>[4x]MNKHVNKVALIGAGFVGSSYAFALINQGITDELVVIDVNKEKAMGDVMDLNHGKAFAPQPVKTSYGTYEDCKDADIVCICAGANQKPGETRLELVEKNLKIFKGIVSEVMASGFDGIFLVATNPVDILTYATWKFSGLPKERVIGSGTTLDSARFRFMLSEYFGAAPQNVCAHIIGEHGDTELPVWSHANVG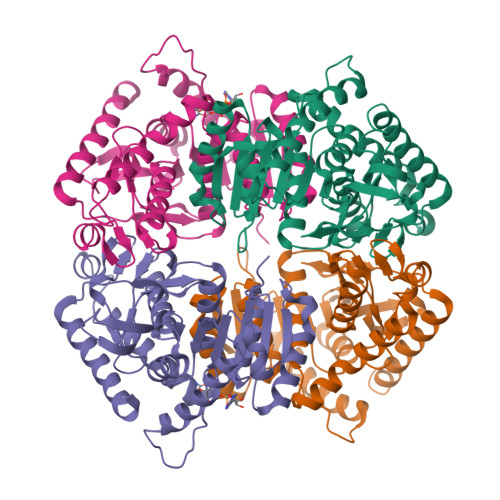GVPVSELVEKNDAYKQEELDQIVDDVKNAAYHIIEKKGATYYGVAMSLARITKAILHNENSILTVSTYLDGQYGADDVYIGVPAVVNRGGIAGITELNLNEKEKEQFLHSAGVLKNILKPHFAEQKVNHHHHHH> GSEELQNKLEDVVIDRNLLILGKILGEGEFGSVMEGNLKQEDGTSLKVAVKTMKLDNSSQREIEEFLSEAACMKDFSHPNVIRLLGVCIEMSSQGIPKPMVILPFMKYGDLHTYLLYSRLETGPKHIPLQTLLKFMVDIALGMEYLSNRNFLHRDLAARNCMLRDDMTVCVADFGLSKKIYSGDYYRQG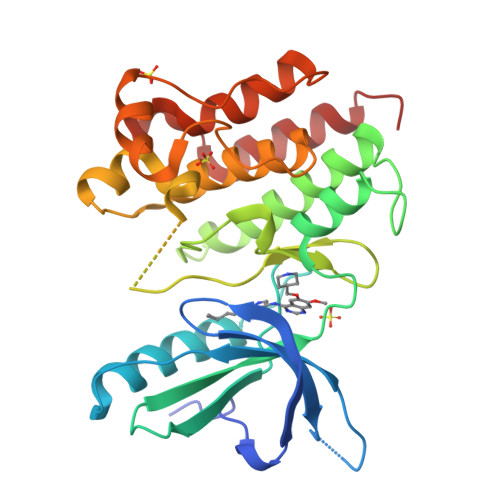RIAKMPVKWIAIESLADRVYTSKSDVWAFGVTMWEIATRGMTPYPGVQNHEMYDYLLHGHRLKQPEDCLDELYEIMYSCWRTDPLDRPTFSVLRLQLEKLLESLPDV>[2x]MSDREFVTVDPVTIIIKECINLSTAMRKYSKFTSQSGVAALLGGGSEIFSNQDDYLAHTFNNLNTNKHNDPFLSGFIQLRLMLNKLKNLDNIDSLTILQPFLLIVSTSSISGYITSLALDSLQKFFTLNIINESSQNYIGAHRATVNALTHCRFEGSQQLSDDSVLLKVVFLLRSIVDSPYGDLLSNSIIYDVLQTILSLACNNRRSEVLRNAAQSTMIAVTVKIFSKLKTIEPVNVNQIYINDESYTNDVLKADTIGTNVESKEEGSQEDPIGMKVNNEEAISEDDGIEEEHIHSEKSTNGAEQLDIVQKTTRSNSRIQAYADDNYGLPVVRQYLNLLLSLIAPENELKHSYSTRIFGLELIQTALEISGDRLQLYPRLFTLISDPIFKSILFIIQNTTKLSLLQATLQLFTTLVVILGNNLQLQIELTLTRIFSILLDDGTANNSSSENKNKPSIIKELLIEQISILWTRSPSFFTSTFINFDCNLDRADVSINFLKALTKLALPESALTTTESVPPICLEGLVSLVD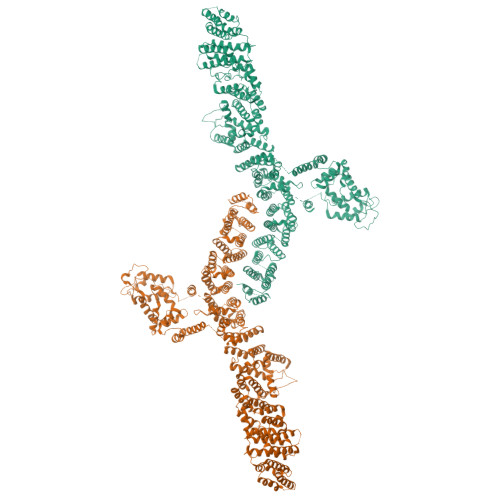DMFDHMKDIDREEFGRQKNEMEILKKRDRKTEFIECTNAFNEKPKKGIPMLIEKGFIASDSDKDIAEFLFNNNNRMNKKTIGLLLCHPDKVSLLNEYIRLFDFSGLRVDEAIRILLTKFRLPGESQQIERIIEAFSSAYCENQDYDPSKISDNAEDDISTVQPDADSVFILSYSIIMLNTDLHNPQVKEHMSFEDYSGNLKGCCNHKDFPFWYLDRIYCSIRDKEIVMPEEHHGNEKWFEDAWNNLISSTTVITEIKKDTQSVMDKLTPLELLNFDRAIFKQVGPSIVSTLFNIYVVASDDHISTRMITSLDKCSYISAFFDFKDLFNDILNSIAKGTTLINSSHDDELSTLAFEYGPMPLVQIKFEDTNTEIPVSTDAVRFGRSFKGQLNTVVFFRIIRRNKDPKIFSKELWLNIVNIILTLYEDLILSPDIFPDLQKRLKLSNLPKPSPEISINKSKESKGLLSTFASYLKGDEEPTEEEIKSSKKAMECIKSSNIAASVFGNESNITADLIKTLLDSAKTEKNADNSRYFEAELLFIIELTIALFLFCKEEKELGKFILQKVFQLSHTKGLTKRTVRRMLTYKILLISLCADQTEYLSKLINDELLKKGDIFTQKFFATNQGKEFLKRLFSLTESEFYRGFLLGNENFWKFLRKVTAMKEQSESIFEYLNESIKTDSNILTNENFMWVLGLLDEISSMGAVGNHWEIEYKKLTESGHKIDKENPYKKSIELSLKSIQLTSHLLEDNNDLRKNEIFAIIQALAHQCINPCKQISEFAVVTLEQTLINKIEIPTNEMESVEELIEGGLLPLLNSSETQEDQKILISSILTIISNVYLHYLKLGKTSNETFLKILSIFNKFVEDSDIEKKLQQLILDKKSIEKGNGSSSHGSAHEQTPESNDVEIEATAPIDDNTDDDNKPKLSDVEKD>[2x]GGGGGGMPILDSDILYLYDAKLTNPNGDPDDENRPRMDSVTGRNLVSDVRLKRYLRDYWLDDGQDIWVRKNEDGTTTDAKSRMSVLLEEYNRTSGQKLSTKE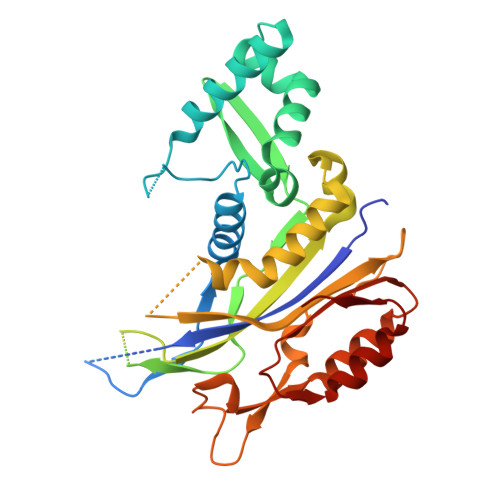ARNSGEFRSWLLDRLMDVRLFGATMPMENSSITFTGPVQFSWGYSLHRVEINNSATISSHFAGRDTEGKGDYGTFGKDWRVLYSLIGFHGIVSRNRARHTGLRESDLEALDRAMLEAIPTEATSRSKIGQIPRFYLRLEYSEGYPYRVGDLREDVVLEPVQGKTLDTLRDVRDYVINLEKVADRIAVRLDGLAGARLYVHPDVTFRGLDSLTGVLGDKLQTLS>HHHHHHMIVLFVDFDYFYAQVEEVLNPSLKGKPVVVCVFSGRFEDSGAVATANYEARKFGVKAGIPIVEAKKILPNAVYLPMRKEVYQQVSSRIMNLLREYSEKIEIASIDEAYLDISDKVRDYREAYNLGL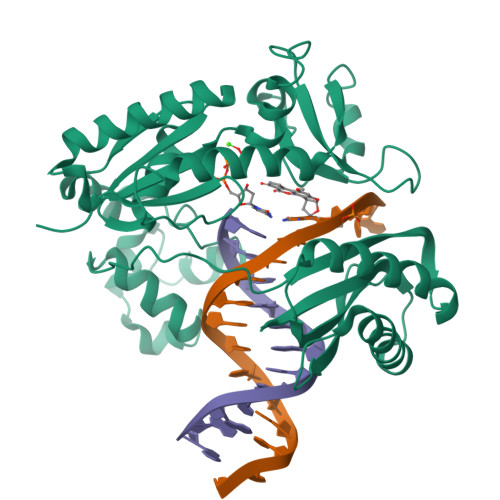EIKNKILEKEKITVTVGISKNKVFAKIAADMAKPNGIKVIDDEEVKRLIRELDIADVPGIGNITAEKLKKLGINKLVDTLSIEFDKLKGMIGEAKAKYLISLARDEYNEPIRTRVRKSIGRIVTMKRNSRNLEEIKPYLFRAIEESYYKLDKRIPKAIHVVAVTEDLDIVSRGRTFPHGISKETAYSESVKLLQKILEEDERKIRRIGVRFSKFI[2x]North-methanocarba-2'-deoxyadenosine triphosphate | C12 H18 N5 O11 P3 | 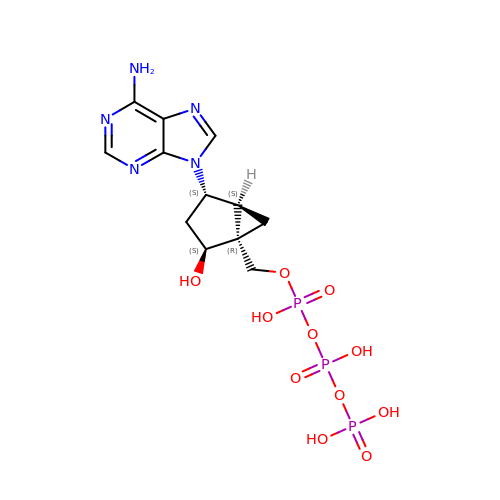ZDQTYRSOYYLILG-VXDIOVFMSA-N Altogether CD38 appears to be a key player in the biosynthesis of calcium messengers which are involved in a wide range of cellular functions. Thus, the catalytic transformation of NAD+ involves the formation, via a ribooxocarbenium ion-like transition state, of a unique reaction intermediate that partitions between several competing pathways such as an irreversible hydrolytic process leading to ADP-ribose and a reversible minor pathway that governs the formation of cADPR. The L-shaped structure of bCD38 consists of two distinct domains separated by a cleft and connected by a hinge region. α-Helices are found mainly in the N-terminal and membrane-proximal domain of this transmembrane protein, whereas β-sheets are preponderant in the distal C-terminal domain. The active site of bCD38 consists in a funnel-shaped cavity with a fairly rigid structure; it buries the NMN+ moiety of the substrate and its scissile bond in its deepest non-polar and least solvent accessible region, whereas the AMP moiety interacts with its more solvent-exposed region, at the entrance of the catalytic cleft.

In agreement with observations on hCD38, incubation of crystals of wt bCD38 with rFNAD and aFNAD resulted in stable covalent intermediates whose structures could be resolved at high resolution. In both complexes, residue Glu218 was found covalently linked to the anomeric carbon C1′ of the fluorinated-ribose ring in an axial (α-anomeric) configuration. Comparison of the covalent complexes obtained with rFNAD and aFNAD allows observing subtle differences that distinguish the way the active site of bCD38 accommodates both ligands. With aFNAD, while one active site (chain A) clearly favors a unique conformation similar to the one observed for rFNAD, the second site reveals the presence of two conformations of the covalently trapped intermediate. It is possible that the fluoride atom in aFNAD slows down the ‘adenine flipping’ described above based on the comparison between the Michaelis complex and the covalent-intermediate obtained with rFNAD. Subtle differences exist, however, within the covalent complexes obtained with aFNAD. Thus, in contrast to chain A (see above), in the chain B of the dimer, the hydrogen bond between the 3′-OH group of the 2′-deoxy-2′-fluoroarabinoside moiety and Oε1 oxygen atom of Glu218 is no longer observed. Furthermore the carboxylate of Glu218 shifts away from the center of the pocket indicating that the conformation of the side chain of the catalytic residue and that of the 2′fluoroarabinoside are particularly affected in the covalent complex with aFNAD. In sharp contrast, the 2′F in the aFNAD covalent intermediate is not involved in any bonding.

>[2x]MADCCTPRKKLCWCVLLFFLVAGITGGAIGIYKWHYSGLNRWHGAGSTADFQKIIQERCDTYTQTIRPGSRSRNCQAIRQAFMSAFISKDPCKATKEDYNSLINLAPPTVPCGQQVFWSKTKELAHEYAKRRRLMTLEDTLLGYLADGLRWCGEPGSSDLNIWSCPDWRKDCRTNYLSVFWEVLSERFAESACNTVRVVLNGSLENAFDSMSIFGRVEAPNLRPQVELEAWLVHDTGKPPSDSCSGSSIRKLKSILDGRNVKFRCMDNLSRDQFLQRS>SLENERLIKMSRFSERGYVVRENGPVYFTKDMDKTVKWFEEILGWSGDIVARDDEGFGDYGCVFDYPSEVAVAHLTPFRGFHLFKGEPIKGVAGFMMIEGIDALHKYVKENGWDQISDIYTQPWGARECSITTTDGCILRFFESIQEG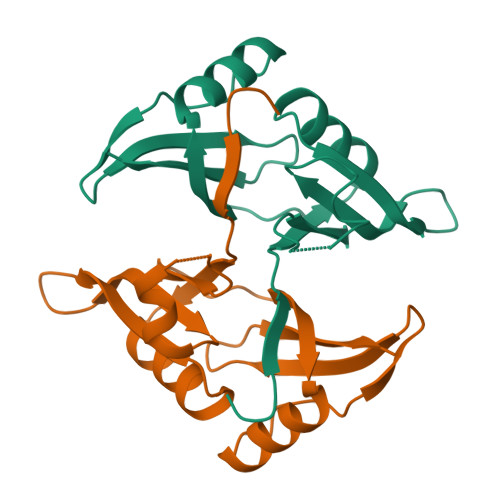[2x]> QGPLGSSEQLKHCNGILKELLSKKHAAYAWPFYKPVDASALGLHDYHDIIKHPMDLSTVKRKMENRDYRDAQEFAADVRLMFSNCYKYNPPDHDVVAMARKLQ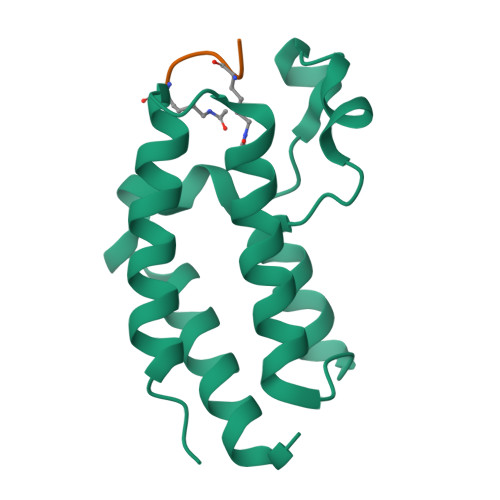DVFEFRYAKMPD;> GGKAGK Trm5a from Pyrococcus abyssi (PaTrm5a) is a newly discovered methyltransferase that catalyses two distinct reactions in tRNA: the N1-methylation of G and the C7-methylation of imG-14 at position 3711. The structural basis of the bifunctional substrate specificity of PaTrm5a is interesting but currently unclear. In this study, we solved the crystal structures of apo-PaTrm5a and PaTrm5a in complex with 5′-methylthioadenosine (MTA), S-adenosyl-L-homocysteine (SAH), and adenosine (ADN) respectively (the chemical structures of these ligands were shown in Supplementary Fig. S1). The 38.5-kDa protein is composed of three domains: D1 (M1-P60), D2 (N70-S162) and D3 (K163-S333). The four structures of PaTrm5a reported in this study all adopt an “open” or extended conformation distinct from that of Trm5b.

To gain more insight into the mechanism of substrate recognition, we soaked or cocrystallised various nucleosides with PaTrm5a and determined the 2.2-Å crystal structure of ADN-bound PaTrm5a, which shows clear ADN density in the map. ADN is recognised by a fashion virtually identical to that of SAH or MTA: the hydrogen bonding network of the adenine ring involves a total of six residues and two well-positioned water molecules, and is further stabilised by the hydrophobic interactions with Ile214, Phe191 and the adenine ring. In PaTrm5a, the OD1 and OD2 atoms of Glu213 in motif 2 form hydrogen bonds with both the O2′ and O3′ hydroxyls of the ribose (left, wheat). The main chain of the Val244 forms a hydrogen bond with the N6 atom of ADN. The general recognition mode of ADN is conserved between PaTrm5a and MjTrm5b with minor local structural differences. A pairwise superposition of the Cα atoms of the ADN-bound MjTrm5b and PaTrm5a gives an overall root-mean-square deviation (RMSD) of 3.0 Å for 211 out of the 333 atoms aligned. However, the RMSD of the D3 domains between the two structures is as low as 0.89 Å (over 100 Cα atoms). The large overall RMSD of the former may be attributed to the completely different D1 position of PaTrm5a, which adopts an extended conformation in all four structures. Compared to the ADN-bound MjTrm5b structure, D1 in PaTrm5a is displaced as far as 80 Å. In the complex structures, the MTA-, SAH- and ADN-binding pockets align well, and the network of hydrogen bonds that stabilises SAM is maintained completely.

> MGSSHHHHHHLEVLFQGPHMSGVKVRREDAKKVLELLKSVGILDGKRKAIRDEKYVIFPVTDTNIAKSLGLEVVDVELPMRPERQIYKNLEDLLPREIFKKLGRLDIVGDIAIVSIPDEILSEREVIVSAIRKLYPKVKVIARRGFHSGLYRIRELEVIWGENRLHTIHKENGVLIKVDLSKVFFNPRMKGERYRIAQLVNDGERILVPFAGVIPYPLVIARFKNVEVYAVEINEFAVKLAEENLELNRDRLKGKIKIIHGDVFEVLPNLPNFDRVVSPTPKGVDALSLTLSKAEKFLHYYDFVHESEIERFRERVLEECRRQGKECRVSVRKVSDYKPHVYKVCADVEILS Peptidase-containing ABC transporters (PCATs) in gram-positive bacteria function both as maturation proteases and exporters for biofilm formation, quorum sensing, or antimicrobial polypeptides. Substrates of PCATs are synthesized as precursors with an N-terminal leader peptide. Proteolytic cleavage of the leader peptide at the conserved double-glycine motif is necessary for secretion of the cargo peptide. In this work, we determined the structures of wild-type PCAT1 (wtPCAT1) in the presence of substrate and ATP with or without Mg2+.

To analyze the conformational states of PCAT1 under ATP turnover conditions, cryo-EM samples were prepared using wtPCAT1 mixed with twofold molar excess of the substrate CtA, 10 mM ATP-Mg2+, and the creatine phosphate ATP-regenerating system. Among the 671,000 particles analyzed by three-dimensional (3D) classification, ∼83% exhibit IF conformations with different degrees of NBD separation, 14% are in an NBD-dimerized configuration, and the remaining 3% do not show any protein features. Subsequent refinement resulted in a low-resolution (6.6-Å) NBD-dimerized structure and three molecular structures of NBD-separated IF conformations, referred to as IF wide (IFW, 4.1 Å), intermediate (IFI, 3.7 Å), and narrow (IFN, 3.7 Å), respectively. The three IF structures share a similar overall conformation, in which the two PEP domains dock symmetrically onto the intracellular openings of the TM cavity. The leader peptide (residues 8 to 24) of the substrate forms an L-shaped structure wrapping around the PEP domain. The double-glycine cleavage site (G23/G24) is positioned on a narrow cleft on PEP in close proximity to the catalytic triad residues C21, H99, and D115. Consistently, the density inside the TM cavity is separated from both leader peptides, indicating that the cargo peptide inside the TM cavity has been freed from its leader peptide. Densities consistent with ATP and Mg2+ were observed in all three reconstructions. Different from the NBD-dimerized structure, in the NBD-separated conformations, ATP binds to the Walker A/B motifs of one NBD, distant from the ABC signature motif of the opposite NBD. The majority of PCAT1 adopts an IF conformation in which the NBDs are separated, the substrate is enclosed inside the TM cavity, and the PEP domains remain associated with the transporter core.

>[2x]SNAMLRRLFKKKYVCVRQYDLTDCGAACLSSIAQYYGLKMSLAKIREMTGTDTQGTNAYGLIHAAKQLGFSAKGVKASKEDLLKDFRLPAIANVIVDNRLAHFVVIYSIKNRIITVADPGKGIVRYSMDDFCSIWTGGLVLLEPGEAFQKGDYTQNMMVKFAGFLKPLKKTVLCIFLASLLYTALGIAGSFYIKFLFDDLIKFEKLNDLHIISAGFAVIFLLQIFLNYYRSILVTKLGMSIDKSIMMEYYSHVLKLPMNFFNSRKVGEIISRFMDASKIRQAISGATLTIMIDTIMAVIGGILLYIQNSSLFFISFIIILLYGIIVTVFNKPIQNANRQIMEDNAKLTSALVESVKGIETIKSFGAEEQTEKSTRDKIETVMKSSFKEGMLYINLSSLTGIVAGLGGIVILWAGAYNVIKGNMSGGQLLAFNALLAYFLTPVKNLIDLQPLIQTAVVASNRLGEILELATEKELREDSDDFVISLKGDIEFRNVDFRYGLRKPVLKNINLTIPKGKTVAIVGESGSGKTTLAKLLMNFYSPEKGDILINGHSIKNISLELIRKKIAFVSQDVFIFSGTVKENLCLGNENVDMDEIIKAAKMANAHDFIEKLPLKYDTFLNESGANLSEGQKQRLAIARALLKKPDILILDEATSNLDSITENHIKDAIYGLEDDVTVIIIAHRLSTIVNCDKIYLLKDGEIVESGSHTELIALKGCYFKMWKQTENTLAS;>SNAMSEAKKLNIGRELTDEELMEMTGGSTFSIQCQKDYTYKPSLPVVKYGVVIDEPEVVIKYGVGPIVGIKYGVEPIGPIQPMYGIKPVETLK[2x]>[2x]AMKNFRLSEKEVKTLAKRIPTPFLVASLDK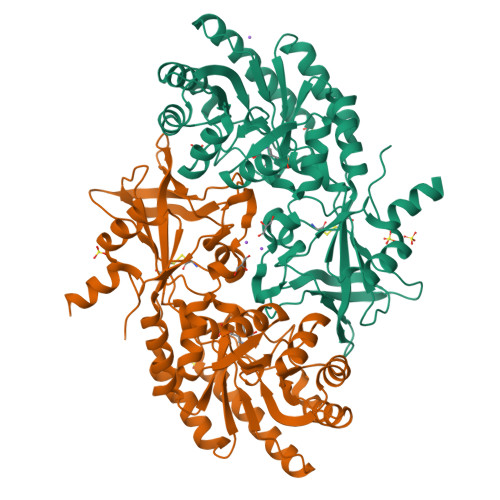VEENYQFMRRHLPRAGVFYAMKANPTPEILSLLAGLGSHFDVASAGEMEILHELGVDGSQMIYANPVKDARGLKAAADYNVRRFTFDDPSEIDKMAKAVPGADVLVRIAVRNNKALVDLNTKFGAPVEEALDLLKAAQDAGLHAMGICFHVGSQSLSTAAYEEALLVARRLFDEAEEMGMHLTDLDIGGGFPVPDCKGLNVDLAAMMEAINKQIDRLFPDTAVWTEPGRYMCGTAVNLVTSVIGTKTRGEQPWYILDEGIYGCFSGIMYDHWCYPLHCFGKGNKKPSTFGGPSCDGIDVLYRDFMAPELKIGDKVLVTEMGSYTSVSATRFNGFYLAPTIIFEDQPEYAARLTEDDDVKKKAAV> MDHHHHHHMKVTIPSGKRYYYAGMGITTPGGKVDIADSKKKSKTRIYTESGWFLSDRAIGQGVSGIVPVGTIGQKGDGTISQTLFPEMPTDFKQLSKLETGIHITDDMRGKYLTFAARAINSYGRVGNYQEADRIWIMGLPVTQNVRLHTDADLALLKNGNTTSLIPTDNQLHTNTEVRDYFNDVVYGATIPVLNYKEPAINQTRQLIALDGRTMQFSNHNFNNGYTTSVLIGNRQQTGPLLTYKLDDTLT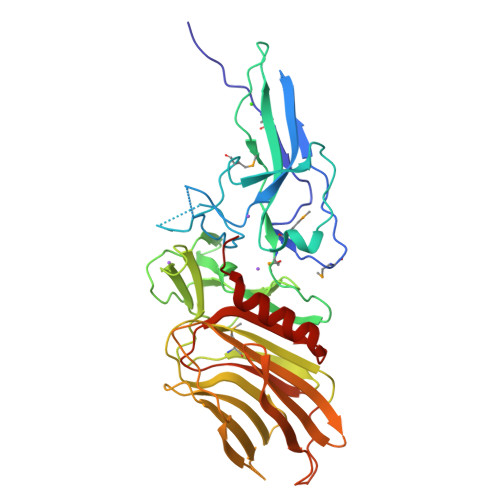WGINLENDGRIAIKTVDTTTANNGGQEYIQNVKLDYSNDNSIQVRSAAKNGSLGIEIFINGQSVYNKTVSLTRNRTTHNISSGQIIFGGNTYINEFAVYTESLNNSNIQKLAEYFRDKYKAS> SMTDTRRRVKVYTLNEDRQWDDRGTGHVSSGYVERLKGMSLLVRAESDGSLLLESKINPNTAYQKQQDTLIVWSEAENYDLALSFQEK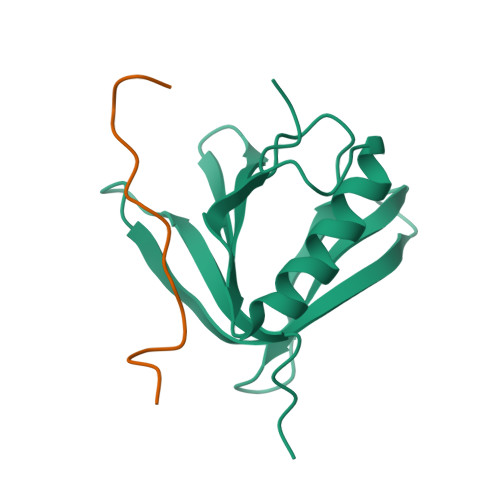AGCDEIWEKICQVQGKDPSVDITQDLVDES;> SLPFTFKVPAPPPSLPPSW Chitin, a linear polymer of β-(1,4) linked N-acetylglucosamine (GlcNAc) forms the rigid inner layer of the cell wall and is also partially hydrolysed during morphogenesis. This is performed by glycoside hydrolase family 18 (GH18) chitinases that catalyse the cleavage of β-(1,4) glycosidic bonds between GlcNAc residues. In contrast, “plant-type” enzymes are predominantly cell wall associated endochitinases. Here we describe the discovery of novel, low micromolar chemical inhibitors of Aspergillus fumigatus family 18 plant-type chitinase A1 (AfChiA1) by high-throughput screening (HTS).

AfChiA1 crystals were soaked with compound 1, diffraction data were collected and scaled to 1.9 Å resolution, the AfChiA1-compound 1 complex structure solved by molecular replacement and refined to an Rfree of 0.22. Electron density corresponding to the ligand (compound 1) was observed in the active site for both molecules in the asymmetric unit. Compound 1 consists of two ring systems, an isoxazolopyrimidine stacking on Trp312 and an attached methoxybenzene. The pyrimidine moiety inserts deeply into the AfChiA active site and thus is likely most important for binding. The 6-methyl of the pyrimidine moiety inserts into a pocket at the bottom of the binding cleft that is formed by Tyr34, Met310, Ala205 and Gln230. Residues lining the AfChiA1 active site form a number of hydrogen bonds with the ligand: the N1 ring atom donates a hydrogen bond to the side chain of Asp172, while the pyrimidine carbonyl group originating from the C2 position accepts a hydrogen bond from the backbone amine of Ala124 and the N5 ring atom accepts a third hydrogen bond from the side chain hydroxyl of Tyr232. The isoxazolo moiety points out of the binding cleft. It forms no direct hydrogen bonds with the protein, but engages in a (weak) water-mediated hydrogen bonding interaction with the side chain amide of Asn233 and the backbone carbonyl of Ala279. The methoxyphenyl moiety makes limited van der Waals contacts with the side chains of Trp312, Gln37, Phe60 and Ala124, but otherwise points towards the bulk solvent suggesting that the ring could be replaced. Strikingly the non-conserved Tyr125 side chain has flipped out to accommodate the methoxy group of the isoxazolo moiety and this may account for the improved inhibition of compound 1 over acetazolamide in AfChiA1 by facilitating tight interactions of the neighbouring pyrimidine moiety within the depths of binding pocket.

>RSNLAIYWGQGPNQLRLSHFCQETSLDIINIGFINYFPDMSPGHWPGSNFGNQCDGSVYVTNDGVVTKLLSGCHQIMEDIPICQAAGKKVLLSIGGAYPPDQSILSEDSAVAFATFLWGAFGPVAEGWEGPRPFGDVVVDGFDFDIEHNGGFGYATMVNTFRQYFNQVPERKFYLSAAPQCIIPDAQLSDAIFNAAFDFIWIQYYNTAACSAKSFIDTSLGTFNFDAWVTVLKASASKDAKLYVGLPASETAANQGYYLTPDEVESLVSTYMDRYPDTFGGIMLWEATASENNQIDGAPYADHMKDILLH[2x]> MNVGDRVRVTSSVVVYHHPEHKKTAFDLQGMEGEVAAVLTEWQGRPISANLPVLVKFEQRFKAHFR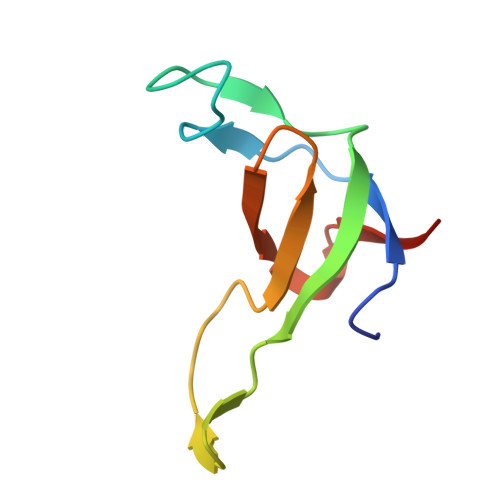PDEVTLIED>MAMRQCAIYGKGGIGKSTTTQNLVAALAEAGKKVMIVGCDPKADSTRLILHSKAQNTIMEMAAEAGTVEDLELEDVLKAGYGDIKCVESGGPEPGVGCAGRGVITAINFLEEEGAYEDDLDFVFYDVLGDVVCGGFAMPIRENKAQEIYIVCSGEMMAMYAANNISKGIVKYANSGGVRLAGLICNSRNTDREDELIMALAEKLGTQMIHFVPRDNVVQRAEIRRMTVIEYDPKAKQADEYRALAQKIIDNKMLVIPTPITMDELEELLMEFGIMDEEDESIVGKTAAEL[3x];> MAMRQCAIYGKGGIGKSTTTQNLVAALAEAGKKVMIVGCDPKADSTRLILHSKAQNTIMEMAAEAGTVEELELEDVLKAGYGDIKCVESGGPEPGVGCAGRGVITAINFLEEEGAYEDDLDFVFYDVLGDVVCGGFAMPIRENKAQEIYIVCSGEMMAMYAANNISKGIVKYANSGGVRLAGLICNSRNTDREDELIMALAEKLGTQMIHFVPRDNVVQRAEIRRMTVIEYDPKAKQADEYRALAQKIIDNKMLVIPTPITMDELEELLMEFGIMDEEDESIVGKTAAEL

Nitrogenase provides access to bioessential nitrogen via the reduction of highly inert atmospheric dinitrogen (N2) to ammonia (NH3). In all nitrogenase isozymes, H-subunits form a homodimeric reductase component (‘HH’) that transiently associates with and transfers electrons to a catalytic core. This catalytic component is a heterotetramer composed of two D- and two K-subunits (‘DDKK’ or α2β2) and contains the active site metallocluster where N2 is bound and reduced to NH3. Three previously characterized ancestral variants were targeted from phylogenetic nodes within the evolutionary lineage of Azotobacter vinelandii Nif (wild-type, ‘WT’) (Garcia et al., 2023): Anc1A, Anc1B, and Anc2.

Anc1B, by contrast, is composed of ancestral H-, D-, and K-subunit proteins. Ancestral variants preferentially bind to the ATP cofactor and exhibit the same general mechanism for N2 binding and reduction conserved across all known nitrogenases to date, but with decreased activity for reduction of N2 or other substrates. Given that most ancestral DDKK substitutions were not close to metalloclusters, we hypothesized that those situated at the DDKK-HH interface might have modified the activity of the ancestors by impeding protein–protein interactions that are necessary for electron transfer to the nitrogenase active site, as well as cofactor loading and complex maturation. Additionally, two unique single-point substitutions in the ancestral K-subunit—K211N and G307N, specific to Anc1B—are likely to impact interactions with HH E111 in the ATP-bound state. Positioned centrally within the DDKK-HH interface, these substitutions alter the electrostatic surface of HH. In Anc1B, the substitution HH S177G is located near the interface with NifDK, with G307N in Anc1B NifK identified as a potential interaction partner.>EPL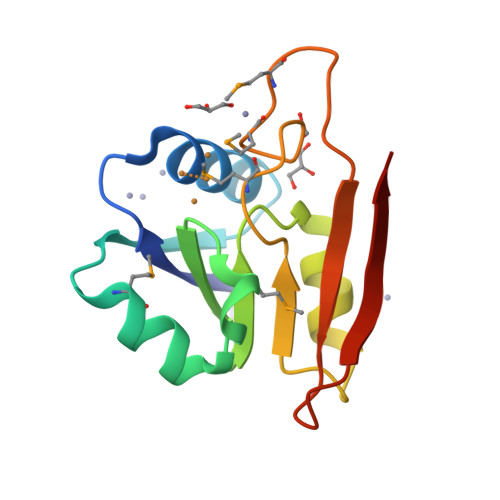AIDVHRDANCGCCKDWIKHLEANGFKVTDHVEADMSAVKSRLGVPYSMGSCHTGVIDGKFVEGHVPAADILKLRERADLVGAAVPGMPVGSPGMEMGDRQDAYQVVGLTRSGQASVLAEYPGR[2x]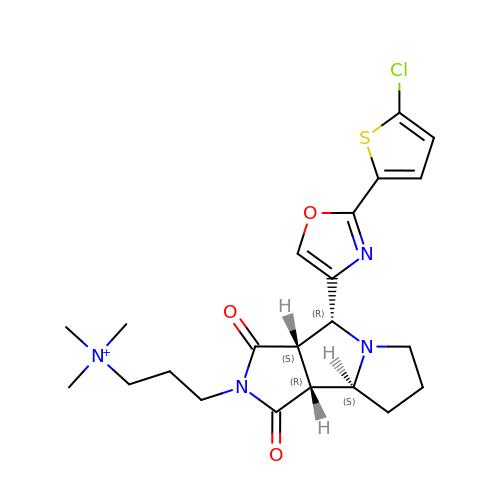3-[(3AS,4R,5S,8AS,8BR)-4-[2-(5-CHLOROTHIOPHEN-2-YL)-1,3-OXAZOL-4-YL]-1,3-DIOXO-4,6,7,8,8A,8B-HEXAHYDRO-3AH-PYRROLO[3,4-A]PYRROLIZIN-2-YL]PROPYL-TRIMETHYL-AZANIUM | C22 H28 Cl N4 O3 S | JCNHSXPHCSYYCR-QZHFEQFPSA-N>[4x]GSSGIVMADWLKIRGTLKSWTK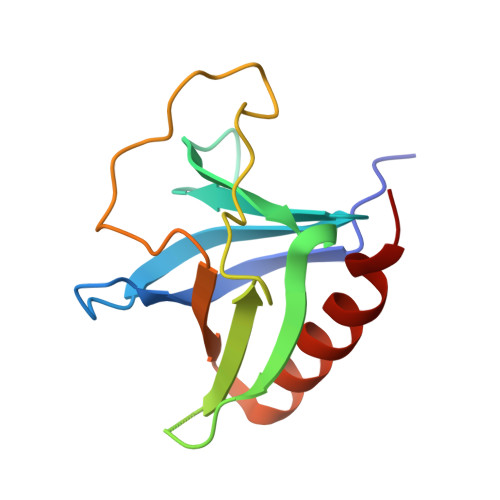LWCVLKPGVLLIYKTQKNGQWVGTVLLNACEIIERPSKKDGFCFKLFHPLEQSIWAVKGPKGEAVGSITQPLPSSYLIIRATSESDGRCWMDALELALKSG> SNADEPQGLFSLGSLESTAAVRIPSTLAHFNQRYPKIHLALSTGPSGTMIDGVLEGALSAAFVDGPLVHPGLEGLPVFPEEMMIVAPYGHAPITRASEVNGANVYAFRANCSYRRHFESWFHADRATPGRIHEMESYHGMLACVIAGAGLALIPRSMLESMPGHQQVSAWPLAEEWRWLTT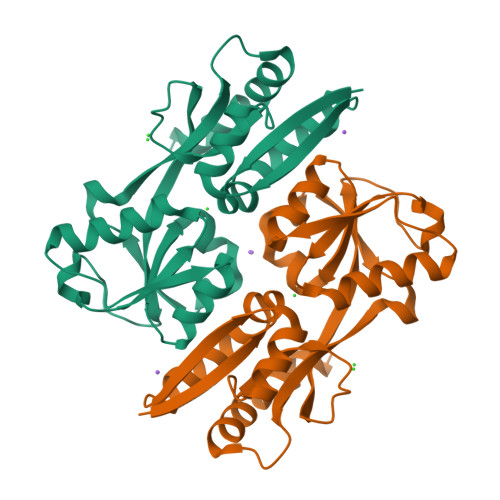WLVWRRGAKTRQLEAFIALLNEDRQTVVSP Pum is a founding member of the Pum/fem-3 mRNA-binding factor (FBF), or PUF family, of eukaryotic RBPs. Pum binds with high affinity to specific sequences in target mRNAs and represses protein expression and enhances mRNA degradation. Regulation of hb mRNA by Pum relies on the spatial distribution of Nos, a tandem CCHC Zn finger (ZF) RBP. Here, we report the crystal structures of Nos-Pum-RNA complexes, which reveal that Nos acts as a molecular clamp that embraces both Pum and RNA.

The Cyclin B (CycB) NRE contains a PRE that diverges from the consensus with uracils in place of adenines at positions +6 and +8, and it has a different NBS sequence. Pum alone did not form a stable complex with CycB NRE RNA (left, and 6B), but remarkably, addition of Nos ZC resulted in ternary complex formation with an apparent Kd of 12 nM (right, and 6B), similar to the 8.7 nM Kd for hb NRE2. To gain molecular insight into how Nos enhances Pum recognition of different NRE sequences, we determined a 4.0 Å crystal structure of a ternary complex with a CycB NRE RNA (5´-UAUUUGUAAUUUAU, core PRE underlined). The protein structures are essentially unchanged compared to the complex with hb NRE2 RNA; however, differences in Pum binding to bases +5 to +8 result in distinct conformations of hb and CycB RNAs in this region (Figure 6C and Figure 6―figure supplement 5). In contrast, Pum appears to bind to the CycB PRE using the 1 repeat:1 RNA base PUF recognition mode with R1271Pum sandwiched between bases +4 and +5. However, for the CycB RNA, recognition of +6U is suboptimal and the +8U nucleotide is disordered in the ternary complex. Thus, Nos stabilizes binding of Pum to RNAs that do not match the PRE consensus sequence in the 3´ half, reducing Pum specificity to allow regulation of a broader range of mRNA targets than Pum alone. Nos and Pum recognize their respective NBS and PRE elements; however, Nos recognition of the 5´ NBS and clamp-like binding to Pum and RNA relaxes the sequence requirements of Pum interaction with the 3´ end of the PRE, as with CycB mRNA, which effectively shifts the recognition sequence, rather than extending it.

> SGRSRLLEDFRNQRYPNLQLRDLANHIVEFSQDQHGSRFIQQKLERATAAEKQMVFSEILAAAYSLMTDVFGNYVIQKFFEFGTPEQKNTLGMQVKGHVLQLALQMYGCRVIQKALESISPEQQQEIVHELDGHVLKCVKDQNGNHVVQKCIECVDPVALQFIINAFKGQVYSLSTHPYGCRVIQRILEHCTAEQTTPILDELHEHTEQLIQDQYGNYVIQHVLEHGKQEDKSILINSVRGKVLVLSQHKFASNVVEKCVTHATRGERTGLIDEVCTFNDNALHVMMKDQYANYVVQKMIDVSEPTQLKKLMTKIRPHMAALRKYTYGKHINAKLEK;> SRGASNSSNNNNNNNKVYKRYNSKAKEISRHCVFCENNNEPEAVINSHSVRDNFNRVLCPKLRTYVCPICGASGDSAHTIKYCPKKPIITMEDAIKAESFRLAKSSYYKQQMKVV> MKRLLLSAAILSSMALFNVNAQELKTSADMKGSFKKNVVLEVFTAEWCGYCPGGKERIAKAIE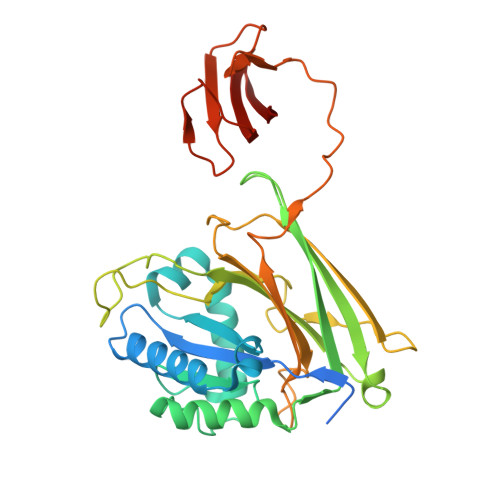MLDDEYKERVFQTFVHYNDGISKKWPRVGQLFIALDQTLGIPGFPTFSVCRMEKKGENLSIGAPIAIKNKIMKGFGDGTAPAEVNLKLTKGATPEDVCTATFTGKVDADLIGKPLMLTAYVLKNNMKPINPQNGAGDGYLHQHTVLMILSTDVKGDALNIAADGSFTIKKEFKLDGFEIKDTDVLAFVHHPMSNAENHSIINAGQESLDKAEPTATEQIVATPSVKAYVQNGKIVVEEEYSKMEVFNATGQLVKNESLVPGVYVVRITANGVMHFLKVLVP> GLPVLNTPGSNQFMTSDDFQSPSAMPQFDVTPHMDIPGEVHNLMEIAEVDSVVPVNNIKANLQS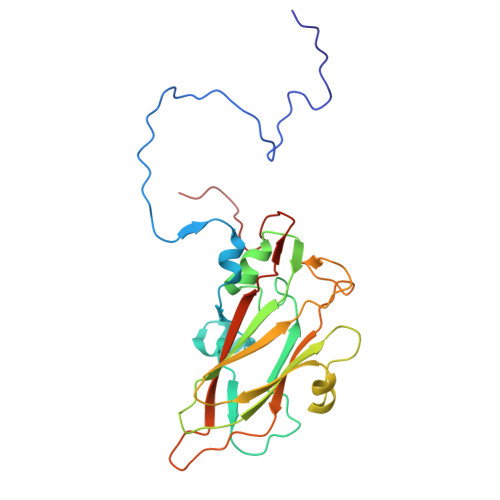MDAYHIEVNTGNYQGEKIFAFQMQPGLESVFKRTLMGEILNYYAHWSGSIKLTFTFCGSAMATGKLLLAYSPPGADVPATRKQAMLGTHMIWDIGLQSSCVLCIPWISQTHYRLVQQDEYTSAGNVTCWYQTGIVVPPGTPNKCVVLCFASACNDFSVRMLRDTPFIGQTALLQ>[6x]SNAMACTGPSLPSAFDILGAAGQDKLLYLKHKLKTPRPGCQGQDLLHAMVLLKLGQETEARISLEALKADAVARLVARQWAGVDSTEDPEEPPDVSWAVARLYHLLAEEKLCPASLRDVAYQEAVRTLSSRDDHRLGELQDEARNRCGWDIAGDPGSIRTLQSNLGCLPPSSALPSGTRSLPRPIDGVSDWSQG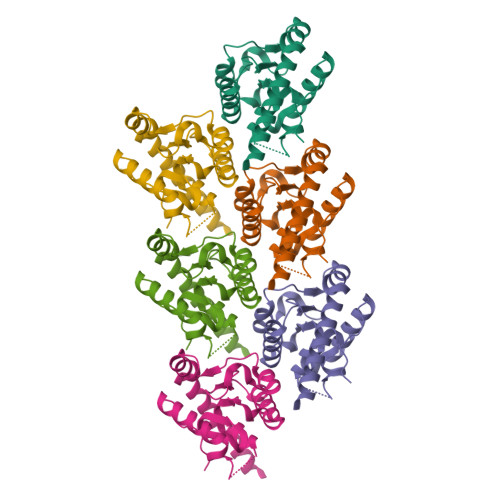CSLRSTGSPASLASNLEISQSPTMPFLSLHRSPHGPSKLCDDPQASLVPEPVPGGCQEPEEMSWPPSGEIASPPELPSSPPPGLPEVAPDATSTGLPDTPAAPETSTNYPVECTEGSAGPQSLPLPILEPVENPCSVKDQTPLQLSVEDTTSPNTKPCPPTPTTPETSPPPPPPPPSSTPCSAHLTPSSLFPSSLESSSEQKFYNFVILHARADEHIALRVREKLEALGVPDGATFCEDFQVPGRGELSCLQDAIDHSAFIILLLTSNFDCRLSLHQVNQAMMSNLTRQGSPDCVIPFLPLESSPAQLSSDTASLLSGLVRLDEHSQIFARKVANTFKPHRLQARKAMWRKEQDTRALREQSQHLDGERMQAAALNAAYSAYLQSYLSYQAQMEQLQVAFGSHMSFGTGAPYGARMPFGGQVPLGAPPPFPTWPGCPQPPPLHAWQAGTPPPPSPQPAAFPQSLPFPQSPAFPTASPAPPQSPGLQPLIIHHAQMVQLGLNNHMWNQRGSQAPEDKTQEAEHHHHHH>GPSFWLGNETLKVPLALFALNRQRLCERLRKNPAVQAGSIVVLQGGEETQRYCTDTGVLFRQESFFHWAFGVTEPGCYGVIDVDTGKSTLFVPRLPASHATWMGKIHSKEHFKEKYAVDDVQYVDEIASVLTSQKPSVLLTLRGVNTDSGSVCREASFDGISKFEVNNTILHPEIVECRVFKTDMELEVLRYTNKISSEAHREVMKAVKVGMKEYELESLFEHYCYSRGGMRHSSYTCICGSGENSAVLHYGHAGAPNDRTIQNGDMCLFDMDGEYYCFASDITCSFPANGKFTADQKAVYEAVLRSSRAVMGAMKPGVWWPDMHRLADRIHLEELAHMGILSGSVDAMVQAHLGAVFMPHGLGHFLGIDVHDVGGYPEGVERIDEPG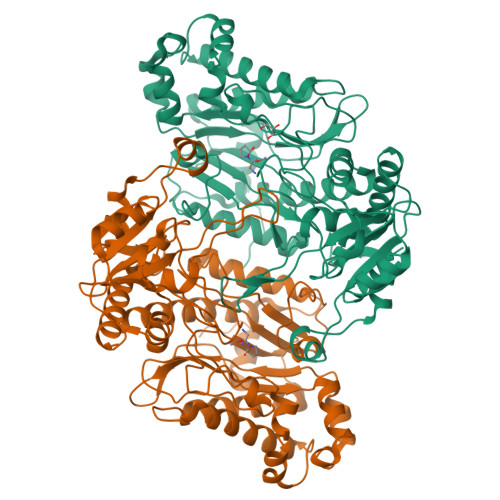LRSLRTARHLQPGMVLTVEPGIYFIDHLLDEALADPARASFLNREVLQRFRGFGGVRIEEDVVVTDSGIELLTCVPRTVEEIEACMAGCDKAFTPFSGPK[2x]>MAHHHHHHGSSEIHLDDLDRNILRLLKKDARLTISELSEQLKKPESTIHFRIKKLQERGVIERYTIILGEQLKPKHLALIVLEVGKPVIEDFLERYISYISSTLSALPGVLFVAKSGEDKIIALVGKNNKDELVKFIEE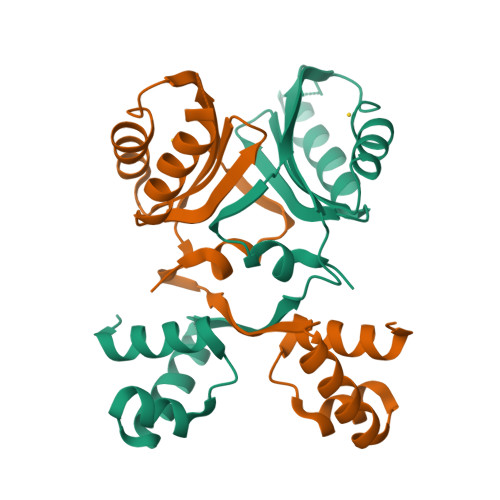NITSIPNLKHIQIFPITEIKKGEDLTGFLAEV[2x]> MKNVGFIGWRGMVGSVLMDRMSQENDFENLNPVFFTTSQAGQKAPVFGGKDAGDLKSAFDIEELKKLDIIVTCQGGDYTNEVYPKLKATGWDGYWVDAASALRMKDDAIIVLDPVNQHVISEGLKKGIKTFVGGNSTVSLMLMAIGGLFEKDLVEWISVATYQAASGAGAKNMRELLSQMGLLEQA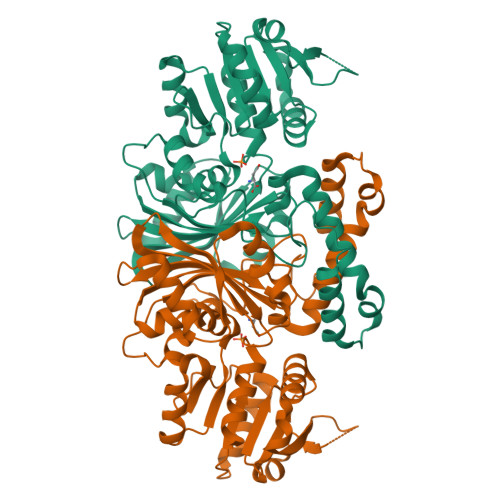VSSELKDPASSILDIERKVTAKMRADNFPTDNFGAALGGSLIPWIDKLLPETGQTKEEWKGYAETNKILGLSDNPIPVDGLCVRIGALRCHSQAFTIKLKKDLPLEEIEQIIASHNEWVKVIPNDKEITLRELTPAKVTGTLSVPVGRLRKLAMGPEYLAAFTVGDQLLWGAAEPVRRILKQLVA>[2x]GSMLDGPYQPTTFTPPSDYWILINSNTNGVVYESTNNSDFWTAVIAVEPHVDPVDRQYNVF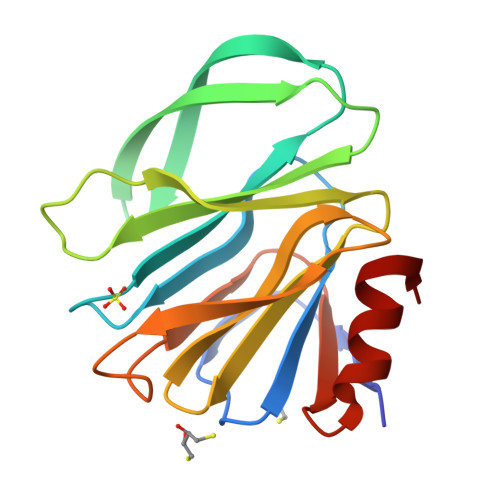GENKQFNVRNDSDKWKFLEMFRGSSQNDFYNRRTLTSNTRLVGILKYGGRIWTFHGETPRATTDSSNTANLNGISITIHSEFYIIPRSQESKCNEYINNGL>[2x]R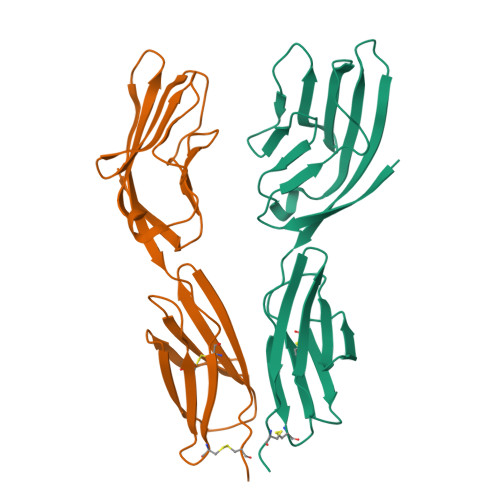DSGTVWGALGHGINLNIPNFQMTDDIDEVRWERGSTLVAEFKRKMKPFLKSGAFEILANGDLKIKNLTRDDSGTYNVTVYSTNGTRILNKALDLRILEMVSKPMIYWECSNATLTCEVLEGTDVELKLYQGKEHLRSLRQKTMSYQWTNLRAPFKCKAVNRVSQESEMEVVNCPE>MSLPLLRPFETVSLENAVEDLVVRFILNVPPEDLSTVERVLFHFEEASWFYTDFVKLMNPYLPNLSIKSFSKIVIDICPLIWNWDITPENALVKFSNYKKTIPVRGAAIFNDSLSKILLLRGINSKHWSFPRGKIGKDEDDVACCIREVKEQTGFDLTGFIDADQYVERNMNGKNFKIFLVKGVPEDFEFKPEHKNEIQAIEWKDFKKLSKAITKNEGSAKVFLVNSMIRPLSLYVKNEKRAKDENKLKLYAEEHLKSILGLNKKENKIVLDAGR[2x];>GSMSTETLEIYRKALNFNVIARYDPKIKQLLFHTPHATVYKWGDDNWNKLEYQGVLAIYLRDVGDKEAILPEVSSYDDTITGQQSEANTPHVLTGHDIYNYGLIIMNRINPDNFSLAIAPNSVLNKRKLFAPNREEELEPMKVEVRDDLVMIKTLKKEVYGIWVHTPEDRQNIYELIKYLLENEP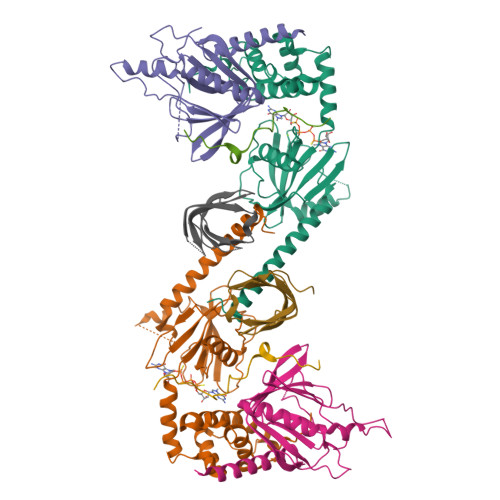TDSFT[2x];>HSKCYAGATFATEAPQVTTLPKPSFV[2x];>MLNFKGYQIEIELKDGKRITGTLKQVSPKSLTLTDAVFQDGGVSPVFKIKADKLYDLKVLKLPPNA[2x]(2~{R})-2-[2-(1~{H}-indol-3-yl)ethylamino]propanoic acid | C13 H16 N2 O2 | 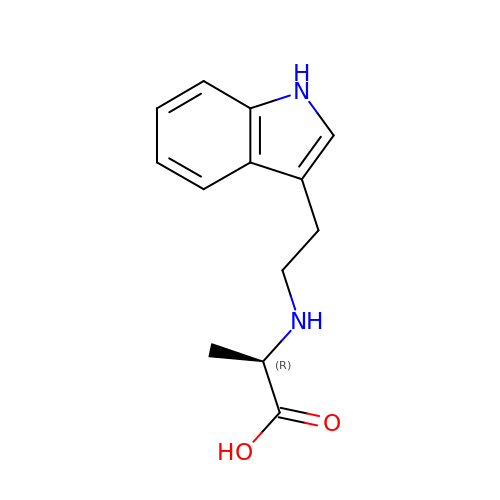BGXZBALMOFWVRC-UHFFFAOYSA-N> MAIIQLPKDFQWGVATAAYQIEGAYNEDGRGLSIWDTFSHTPGKVRNGDNGDIACDSYHRYKEDIKLMKELGVDIYRFSISWPRIFPTGRGPVNSKGLEFYHHFVDELIANGIEPMCTLYHWDLPQSLQDIGGWANREVVEAFVEYSTFIFKEFNGKIKKWITINEPWCISFLSNYEGKHAPGNHNLQLAVTISHHLLLAHGKAVKAFRNLGIEGEIGYAPNVEWIEPFSSKQEDQDACHRGMGIFIEWFFDPVFKGKYPDFMLDWFEQNGAVPEIQEGDMQMISQPIDFVGINFYTGSVGRYNKEAGLLEVEKINIGYQTTDIGWNIYPEGFYKVLNKINNQYGNIPIYITENGACYNDEVINGRVKDEGRIEYLKQHLTSIRRSIETGVNIKGYFAWSLLDNFEWAEGYDMRFGLVHINFHTLERTKKDS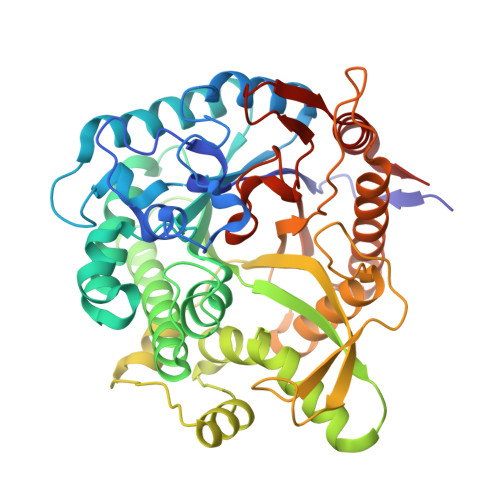YYWYKKIVRNRWFEI> RKIPKVGHTFFQKPESCPPVPGGSMKLDIGIINENQRVSMSRNIESRSTSPWNYTVTWDPNRYPSEVVQAQCRNLGCINAQGKEDISMNSVPIQQETLVVRRKHQGCSVS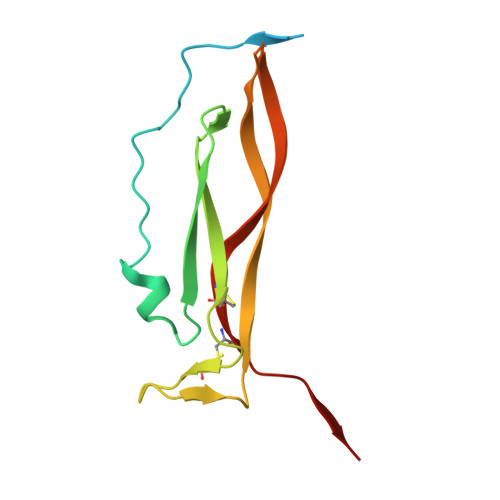FQLEKVLVTVGCTCVTPVIHHVQ2-[(1S)-2-acetyl-1,2-dihydroisoquinolin-1-yl]-N,N-dimethylacetamide 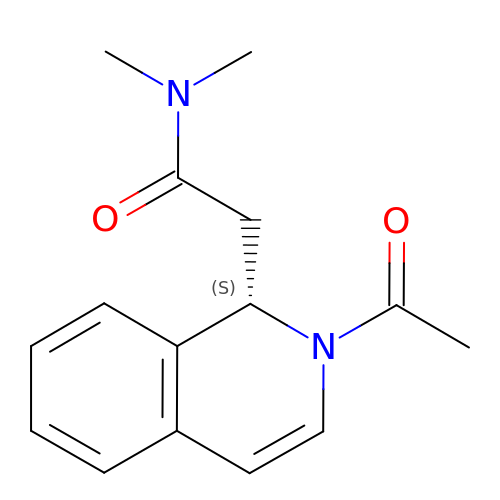| C15 H18 N2 O2 | FYMMJTVLNAKHEX-AWEZNQCLSA-N>GPLGSPEFSKRSSDPSPAGDNEIERVFVWDLDETIIIFHSLLTGTFASRYGKDTTTSVRIGLMMEEMIFNLADTHLFFNDLEDCDQIHVDDVSSDDNGQDLSTYNFSADGFHSSAPGANLCLGSGVHGGVDWMRKLAFRYRRVKEMYNTYKNNVGGLIGTPKRETWLQLRAELEALTDLWLTHSLKALNLINSRPNCVNVLVTTTQLIPALAKVLLYGLGSVFPIENIYSATKTGKESCFERIMQRFGRKAVYVVIGDGV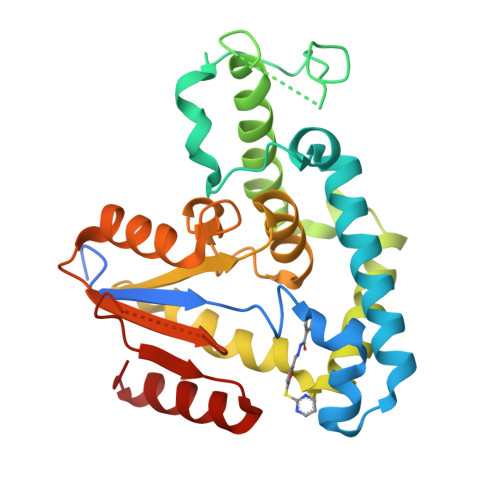EEEQGAKKHNMPFWRISCHADLEALRHALELEYL[3x]> EDELYRQSLEIISRYLREQATGAKDTKPMGRSGATSRKALETLRRVGDGVQRNHETAFQGMLRKLDIKNEDDVKSLSRV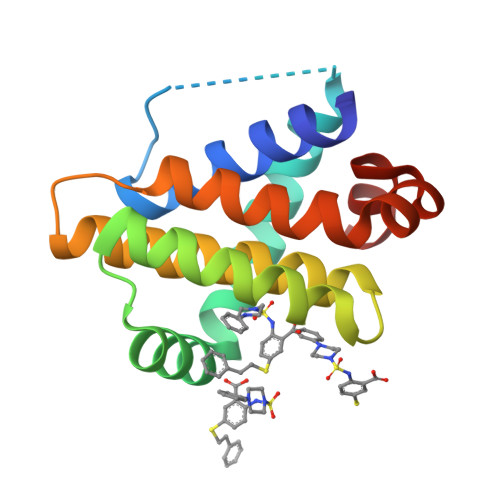MIHVFSDGVTNWGRIVTLISFGAFVAKHLKTINQESCIEPLAESITDVLVRTKRDWLVKQRGWDGFVEFFH> MFRL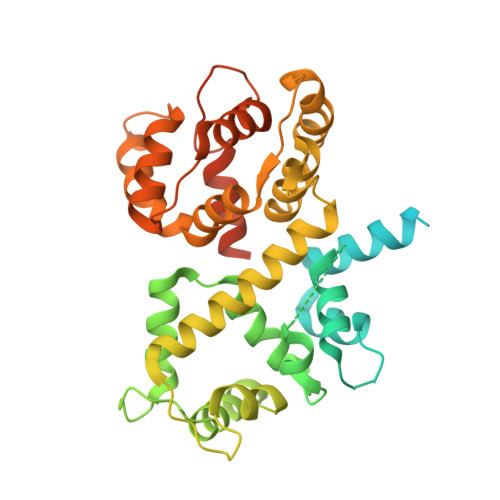NSLSALAELAVGSRWYHGGSQPIQIRRRLMMVAFLGASAVTASTGLLWKRAHAESPPCVDNLKSDIGDKGKNKDEGDVCNHEKKTADLAPHPEEKKKKRSGFRDRKVMEYENRIRAYSTPDKIFRYFATLKVISEPGEAEVFMTPEDFVRSITPNEKQPEHLGLDQYIIKRFDGKKISQEREKFADEGSIFYTLGECGLISFSDYIFLTTVLSTPQRNFEIAFKMFDLNGDGEVDMEEFEQVQSIIRSQTSMGMRHRDRPTTGNTLKSGLCSALTTYFFGADLKGKLTIKNFLEFQRKLQHDVLKLEFERHDPVDGRITERQFGGMLLAYSGVQSKKLTAMQRQLKKHFKEGKGLTFQEVENFFTFLKNINDVDTALSFYHMAGASLDKVTMQQVARTVAKVELSDHVCDVVFALFDCDGNGELSNKEFVSIMKQRLMRGLEKPKDMGFTRLMQAMWKCAQETAWDFALPKQ> MYVRISGRIRLNAHSLNAQGGGGTNYIEITKTKVTVRTENGWTVVEVPAITGNMLKHWHFVGFVDYFKTTPYGVNLTERALRYNGTR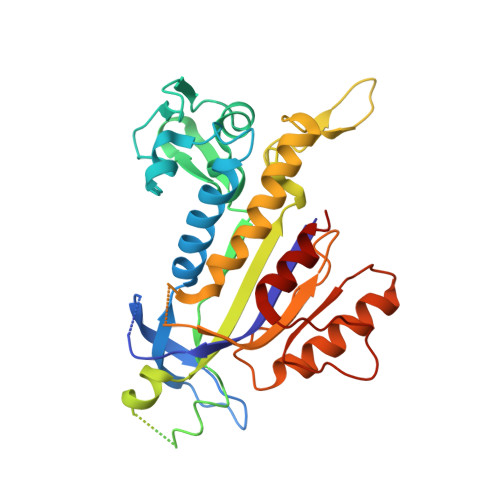FGQGETTATKANGATVQLNDEATIIKELADADVHGFLAPKTGRRRVSLVKASFILPTEDFIKEVEGERLITAIKHNRVDVDEKGAIGSSKEGTAQMLFSREYATGLYGFSIVLDLGLVGIPQGLPVKFEENQPRPNIVIDPNERKARIESALKALIPMLSGYIGANLARSFPVFKVEELVAIASEGPIPALVHGFYEDYIEANRSIIKNARALGFNIEVFTYNVDLGEDIEATKVSSVEELVANLVKMVGGKE>[14x]YILPSFIEHSSFGVKESNPYNKLFEERIIFLGVQVDDASANDIMAQLLVLESLDPDRDITMYINSPGGGFTSLMAIYDTMQYVRADIQTVCLGQAASAAAVLLAAGTPGKRMALPNARVLIHQPSLSGVIQGQFSDLEIQAAEIERMRTLMETTLARHTGKDAGVIRKDTDRDKILTAEEAKDYGIIDTVLEYRKLS;>LTDSVYERLLSERIIFLGSEVNDEIANRLCAQILLLAAEDASKDISLYINSPGGSISAGMAIYDTMVLAPC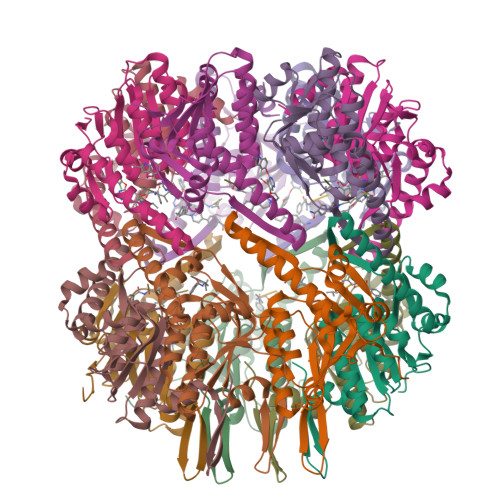DIATYAMGMAASMGEFLLAAGTKGKRYALPHARILMHQPLGGVTGSAADIAIQAEQFAVIKKEMFRLNAEFTGQPIERIEADSDRDRWFTAAEALEYGFVDHIITR[14x]> GAMGSGIQRPSAVTSMTRTRDVMQLWSLLEACLQSNLMKRAFSILESLYLVPEHKQRFIEDYNMYLNSFSKNDPNFPILKMNEKLTNDLETSFKDVNYNDKTLAIMIHHALNFHSTTSSMLLKPIISAYLKMSVNGIREIFSCLDILTISDLNILMNDLKVITPSQLPNSVRPILESLTLSPTPVNNIENEEGLNKVEAENDSKLHKASNASSDSIKKPSLDPLREVSFHGSTEVLSKDAEKLIAVDTIGMRVIRHTLLGLSLTPEQKEQISKFKFDANDNVLKMKPTKNDDNNNSINFFEIYNSLPTLEEKKAFESALNIFNQDRQKVLENRATEAARERWKHDFEEAKARGDISIEKNLNVKLWKWYNEMLPLVKEEINHCRSLLSEKLSDKKGLNKVDTNRLGYGPYLTLIDPGKMCVITILELLKLNSTGGVIEGMRTARAVISVGKAIEMEFRSEQVLKSESQAFRDVNKKSPEFKKLVQNAKSVFRSSQIEQSKILWPQSIRARIGSVLISMLIQVAKVSVQGVDPVTKAKVHGEAPAFAHGYQYHNGSKLGVLKIHKTLIRQLNGERLIASVQPQLLPMLVEPKPWVNWRSGGYHYTQSTLLRTKDSPEQVAYLKAASDNGDIDRVYDGLNVLGRTPWTVNRKVFDVVSQVWNKGEGFLDIPGAQDEMVLPPAPPKNSDPSILRAWKLQVKTIANKFSSDRSNRCDTNYKLEIARAFLGEKLYFPHNLDFRGRAYPLSPHFNHLGNDMSRGLLIFWHGKKLGPSGLKWLKIHLSNLFGFDKLPLKDRVAFTESHLQDIKDSAENPLTGDRWWTTADKPWQALATCFELNEVMKMDNPEEFISHQPVHQDGTCNGLQHYAALGGDVEGATQVNLVPSDKPQDVYAHVARLVQKRLEIAAEKGDENAKILKDKITRKVVKQTVMTNVYGVTYVGATFQIAKQLSPIFDDRKESLDFSKYLTKHVFSAIRELFHSAHLIQDWLGESAKRISKSIRLDVDEKSFKNGNKPDFMSSVIWTTPLGLPIVQPYREESKKQVETNLQTVFISDPFAVNPVNARRQKAGLPPNFIHSLDASHMLLSAAECGKQGLDFASVHDSYWTHASDIDTMNVVLREQFIKLHEVDLVLRLKEEFDQRYKNYVKIGKLKRSTDLAQKIIRIRKDLSRKLGRSTTLADEIYFEKKRQELLNSPLIEDRNVGEKMVTTVSLFEDITDLDALELENGGDENSGMSVLLPLRLPEIPPKGDFDVTVLRNSQYFFS;> MGGSHHHHHHGMASSVPIPGIKDISKLKFFYGFKYLWNPTVYNKIFDKLDLTKTYKHPEELKVLDLYPGVGIQSAIFYNKYCPRQYSLLEKRSSLYKFLNAKFEGSPLQILKRDPYDWSTYSNLIDEERIFVPEVQSSDHINDKFLTVANVTGEGSEGLIMQWLSCIGNKNWLYRFGKVKMLLWMPSTTARKLLARPGMHSRSKCSVVREAFTDTKLIAISDANELKGFDSQCIEEWDPILFSAAEIWPTKGKPIALVEMDPIDFDFDVDNWDYVTRHLMILKRTPLNTVMDSLGHGGQQYFNSRITDKDLLKKCPIDLTNDEFIYLTKLFMEWPFKPDILMDFVDMYQTEHSG

Mitochondrial RNAP (mtRNAP) is essential for mitochondrial DNA transcription and replication in eukaryotes. Mitochondria recruit a single-subunit RNAP and one or two auxiliary factors to initiate transcription. Here we provide a comprehensive, stepwise mechanism of transcription initiation by solving high-resolution cryogenic electron microscopy (cryo-EM) structures of yeast mitochondrial RNAP and the transcription factor Mtf1 catalysing two- to eight-nucleotide RNA synthesis at single-nucleotide addition steps. The Mtf1 is positioned on the top of the polymerase cleft like a lid.

The downstream cleft starts opening in IC3 and continues to open further in IC4; the positions of y-mtRNAP and Mtf1 in IC4 align with those in PmIC. As the RNA–DNA hybrid grows in size from IC2 to IC3 to IC4, the template nucleotides from −4 to −1 are increasingly scrunched. This template scrunching is highest in IC4 among the three states, yet IC4 is substantially less abortive, suggesting that template scrunching is not the primary contributor to the dissociation of 2- and 3-nt RNAs. Notably, the NT strand scrunches in IC2 and IC3 into tight loops and relaxes in IC4. In IC4, the NT strand (+1 to +4) has a poor density and no noteworthy interactions with protein atoms. The NT strand in IC4 carries less stress energy and favours RNA extension over abortive synthesis. Notably, the 4-bp RNA–DNA duplex in IC4 is in a half-translocated state; that is, the 3′ end of the nascent RNA has moved by about 3.5 Å at the C1′ position from the N site but has not reached the P site. No stable PmIC or other intermediate state was observed coexisting in the IC4 cryo-EM sample.>EHAERLPYDASKWEFPRDRLKLGKPLGRGAFGQVIEADAFGIDKTATCRTVAVKMLKEGATHSEHRALMSELKILIHIGHHLNVVNLLGACTKPGGPLMVITEFCKFGNLSTYLRSKRNEFVPYKVAPEDLYKDFLTLEHLICYSFQVAKGMEFLASRKCIHRDLAARNILLSEKNVVKICDFGLARDIYKDPDYVRKGDARLPLKWMAPETIFDRVYTIQSDV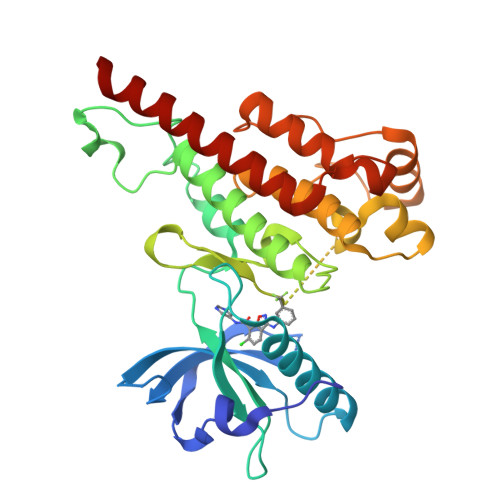WSFGVLLWEIFSLGASPYPGVKIDEEFCRRLKEGTRMRAPDYTTPEMYQTMLDCWHGEPSQRPTFSELVEHLGNLLQANAQQDRHHHHHH[2x]> AAVTRAASASPAPGTGATPDGFSAEESLEEIDGAVSPGPSDAPDGEYGDLDARTAVRAAATERDRFYVCPPPSGSTVVRLEPEQACPEYSQGRNFTEGIAVLFKENIAPHKFKAHIYYKNVIVTTVWSGSTYAAITNRFTDRVPVPVQEITDVIDRRGKCVSKAEYVRNNHKVTAFDRDENPVEVDLRPSRLNALGTRGWHTTNDTYTKIGAAGFYHTG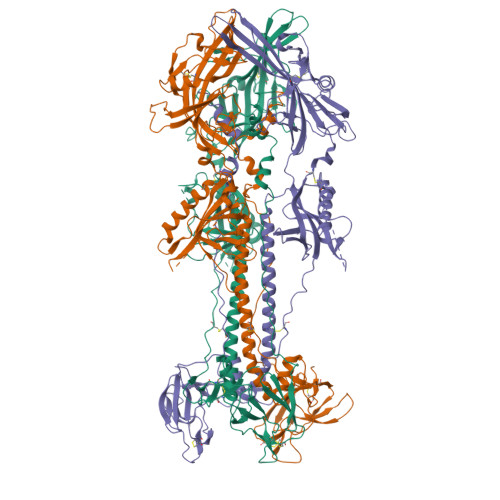TSVNCIVEEVEARSVYPYDSFALSTGDIVYMSPFYGLREGAHGEHIGYAPGRFQQVEHYYPIDLDSRLRASESVTRNFLRTPHFTVAWDWAPKTRRVCSLAKWREAEEMIRDETRDGSFRFTSRALGASFVSDVTQLDLQRVHLGDCVLREASEAIDAIYRRRYNNTHVLAGDKPEVYLARGGFVVAFRPLISNELAQLYARELERLGLAGVVGPASPAAARRARRSPGPAGTPEPPAVNGTGHLRITTGSAEFARLQFTYDHIQAHVNDMLSRIAAAWCELQNKDRTLWGEMSRLNPSAVATAALGQRVSARMLGDVMAISRCVEVRGGVYVQNSMRVPGERGTCYSRPLVTFEHNGTGVIEGQLGDDNELLISRDLIEPCTGNHRRYFKLGGGYVYYEDYSYVRMVEVPETISTRVTLNLTLLEDREFLPLEVYTREELADTGLLDYSEIQRRNQLHALKFYDIDRVVKVDHNHHHHHHHH>MNAAAVTPPPEKFNFAEHLLQTNRVRPDKTAFVDDISSLSFAQLEAQTRQLAAALRAIGVKREERVLLLMLDGTDWPVAFLGAIYAGIVPVAVNTLLTADDYAYMLEHSRAQAVLVSGALHPVLKAALTKSDHEVQRVIVSRPAAPLEPGEVDFAEFVGAHAPLEKPAATQADDPAFWLYSSGSTGRPKGVVHTHANPYWTSELYGRNTLHLREDDVCFSAAKLFFAYGLGNALTFPMTVGATTLLMGERPTPDAVFKRWLGGVGGVKPTVFYGAPTGYAGMLAAPNLPSRDQVALRLASSAGEALPAEIGQRFQRHFGLDIVDGIGSTEMLAAFLSNLPDRVRYGTTGWPVPGYQIELRGDGGGPVADGEPGDLYIHGPSSATMYWGNRAKSRDTFQGGWTKSGDKYVRNDDGSYTYAGRTDDMLKVSGIYVSPFEIEATLVQHPGVLEAAVVGVADEHGLTKPKAYVVPRPGQTLSETELKTFIKDRLAPYKYPRSTVFVAELPKTATGKIQRFKLREGVLG[2x]

BadA catalyzes the conversion of benzoate to benzoyl-CoA in the metabolism of aromatic carboxylic acids. Its catalytic mechanism is shown as follows: benzoate firstly docks to the active site, where it orientates to allow the carboxylic group access to adenosine triphosphate (ATP) for the formation of an adenosine monophosphate (AMP) intermediate; coenzyme A (CoA) subsequently comes in to substitute the AMP-activated intermediate resulting in the formation of benzoyl-CoA. The solved structures show that the benzoate binding cavity is rather small and narrow, constituted by several bulky amino acid residues including Y228, G327, S328, T329, H333, and I334. With the purpose to allow acceptance of various bulkier substrates into the active site, a double mutant H333A and I334A was created.

The mutant was examined against a series of carboxylic acids. To our surprise, most of the tested carboxylic acids can be taken by the mutant to form corresponding CoA products as opposed to the wild type that cannot accept them. There is no significant conformational change between the wild type and the mutant as the root-mean-square deviation for the 394 Cα is about 0.3 Å. Superposition of these residues and ligands for the wild type and the mutant BadA reveals that the overall architecture is almost identical except that the volume of the substrate-binding pocket is increased by 96.7 Å3 in the mutant. Three protein crystal structures in an apo form and in complex with a 2-methylthiazole-5-carboxyl-AMP or 2-choloro-1,3-thiazole-5-carboxyl-AMP intermediate validated the engineering rationality and synthetic practicality of the modified enzyme. BadA that underwent structure-guided protein engineering has clearly exhibited an additional dimension on substrate tolerance in light of 13 novel carboxyl CoA derivatives synthesized herein.>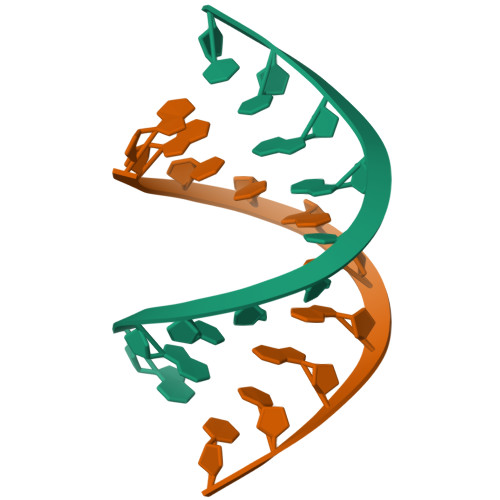 GGCCGCGGCC> HHHVPLTFDLPFEELLTYPGRTPRPADHDEYWDRGLADLAAVPADVVIEPAEFTTPLARCSHLWFTGTGGVRVHAKLLRPVAPVEPHPALLQFHGYTGNSGDWSSRLHYVALGYTVAALDCRGQAGLSVGEAPVENWSMASYLLRGIDDDAADNLALRHLFLDTARLAQIVLAMDDVDPDRVAATGYSQGGGLTLACAALEPRIRLAAPVYPFLCDFRRAWEMDLEKGPYNEITTYFRARDPRHLREEEIFSRLGYVDVQHLAPRVRAEVLMTVSLADKICPPSTQFAAYNKLGGPKDYRLYPDFAHETLPGTDDAIFTFLQGL;>[4x]HVPLTFD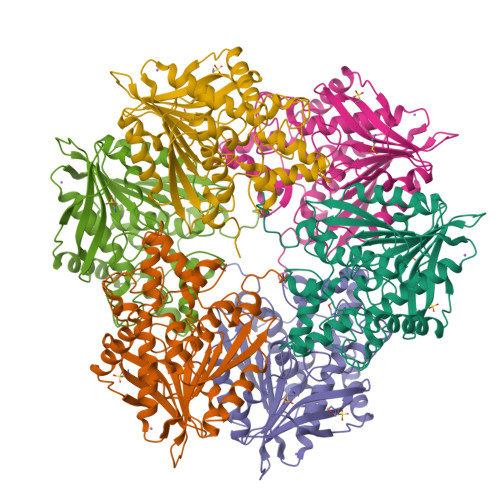LPFEELLTYPGRTPRPADHDEYWDRGLADLAAVPADVVIEPAEFTTPLARCSHLWFTGTGGVRVHAKLLRPVAPVEPHPALLQFHGYTGNSGDWSSRLHYVALGYTVAALDCRGQAGLSVGEAPVENWSMASYLLRGIDDDAADNLALRHLFLDTARLAQIVLAMDDVDPDRVAATGYSQGGGLTLACAALEPRIRLAAPVYPFLCDFRRAWEMDLEKGPYNEITTYFRARDPRHLREEEIFSRLGYVDVQHLAPRVRAEVLMTVSLADKICPPSTQFAAYNKLGGPKDYRLYPDFAHETLPGTDDAIFTFLQGL;> LTFDLPFEELLTYPGRTPRPADHDEYWDRGLADLAAVPADVVIEPAEFTTPLARCSHLWFTGTGGVRVHAKLLRPVAPVEPHPALLQFHGYTGNSGDWSSRLHYVALGYTVAALDCRGQAGLSVGEAPVENWSMASYLLRGIDDDAADNLALRHLFLDTARLAQIVLAMDDVDPDRVAATGYSQGGGLTLACAALEPRIRLAAPVYPFLCDFRRAWEMDLEKGPYNEITTYFRARDPRHLREEEIFSRLGYVDVQHLAPRVRAEVLMTVSLADKICPPSTQFAAYNKLGGPKDYRLYPDFAHETLPGTDDAIFTFLQGL In contrast to the multiple CCD paralogs found in vertebrates, most insect genomes encode a single CCD known as Neither Inactivation Nor Afterpotential B (NinaB). Later studies demonstrated that NinaB not only cleaves carotenoids symmetrically but also isomerizes one-half of its substrate to form a ~1:1 mixture of 11-cis and all-trans RAL products. This enzyme was thus termed an isomerooxygenase. In NinaB, similar to other oxygenase members of the CCD superfamily, the ferrous iron cofactor activates dioxygen for reaction with a target alkene bond within the substrate.

To bridge this gap in understanding, we report a high-resolution crystal structure of NinaB from the cabbage looper (Trichoplusia ni), revealing the molecular architecture of its active site and details of its membrane-interacting structural elements. The structure was solved by molecular replacement in space group C2, revealing an asymmetric unit composed of eight copies of TnNinaB. TnNinaB adopts the classical seven-bladed β-propeller CCD fold with its iron cofactor coordinated at the propeller axis. The NinaB iron center is coordinated by four conserved His residues and contains an additional solvent molecule bound trans to His184. The iron center abuts an extended pocket, ~30 Å in length, that runs along the top face of the β-propeller forming the substrate-binding cleft of the enzyme. As compared with the apocarotenoid-cleaving enzyme NdCCD, the proximal active site size of NinaB is much larger owing to the need to accommodate passage of a β-ionone or 3-hydroxy-β-ionone ring during substrate binding. Other noteworthy features of the active site include the observation of multiple rotamers for Trp17 and Met339, both located in the distal active site, as well as the presence of 2-methyl-2,4-pentanediol (MPD) derived from the crystallization precipitant, which inhibits TnNinaB activity toward zeaxanthin with an half-maximum inhibitory concentration (IC50) value of 0.67% v/v. In the TnNinaB crystal structure, three of the protomers in the asymmetric unit (chains B, F and H) exhibited well-defined density for the entire region while three others had partially resolved sequences (chains D, E and G). Residues 118–126 form a variable-length α-helical structure with pronounced amphipathicity. In both cases, 11-cis isomer production was nearly abolished despite robust oxygenase activity as evidenced by WT-level formation of the all-trans isomer product. Mapping Trp17, Phe357 and the other residues impacting 11-cis formation within the TnNinaB active site revealed their clustering within the distal region of the active site pocket.

>[8x]MAATEEKLYPNCDATVWLRSCEEEVSEPLEGTMTGEFPSWLRGTLLRNGPGCLNVGTMRFEHLFDSSALLHRFAIDDGTVTYQCRFLRTNTLKKNRAANRIVVTEFGTKSAPDPCHTIFDRVAAFFNPGEHMSDNAMISVYPFGDEVYAFTEGPIIHRVDTVTLDTLEQKNMTDCVALVNHTSHPHVMPNGDVYNVGMSVVKGRIRHVVAKFPFTEKGDMFKSAHIVASMAPRWALHPAYMHTFGITENYFVIVEQPLSISVYGLMTNLINNNKLAASLKWYPEYETHIVLLSRTTGKEVKRFRTDTLFFLHIINCYEHEGELVVDLCTYKDAKVVDAMYVHAIETMQSNADYAEWFRAKPKRLQVSLNAPKMTRMKSSILADIGCETPRIHYDLHNSKYYRYFYAISSDVDAENPGTVIKVDTKTGETKTWCRPNCYPSEPIFVPSPNAKDEDDGVLLSALVWGGEMNQTVALLVLNAKTMEEMGRATFNTPSPAPKCLHGWFLPTNG>[2x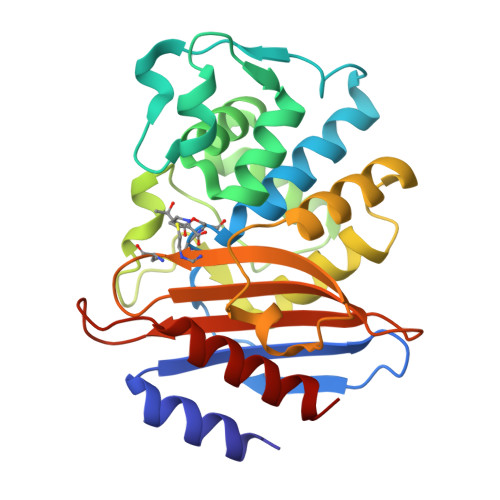]VAEPFAKLEQDFGGSIGVYAMDTGSGATVSYRAEERFPLCSSYKGFLAAAVLARSQQQAGLLDTPIRYGKNALVPWSPISEKYLTTGMTVAELSAAAVQYSDNAAANLLLKELGGPAGLTAFMRSIGDTTFRLDRWELELNSAIPGDARDTSSPRAVTESLQKLTLGSALAAPQRQQFVDWLKGNTTGNHRIRAAVPADWAVGDKTGTCGVYGTANDYAVVWPTGRAPIVLAVYTRAPNKDDKHSEAVIAAAARLALEGL Lassa virus (LASV) nucleoprotein (NP) is the only known 3′-5′ exoribonuclease that can suppress type I interferon (IFN) production possibly by degrading immune-stimulatory RNAs. NP is a multifunctional protein involved in viral genomic RNA encapsidation, viral RNA synthesis, and immune evasion. Our structural, biochemical, and cell-based analyses have demonstrated that NP encodes a functional 3′-5′ exoribonuclease of the DEDDH family at its C terminus and that this RNase activity plays a strikingly important role in IFN suppression. We therefore propose a novel immune evasion mechanism in which NP suppresses the IFN induction by selectively degrading these immune-stimulatory RNAs.

We have also conducted a time course soaking experiment to explore the kinetic process of the LASV NP exoribonuclease function. To do this, we set up a time course experiment to capture the conformational changes of the NP-C·dsRNA complex during the enzymatic reaction. The LASV NP-C·dsRNA complex was soaked in a cryoprotectant solution with 100 mm MnCl2, and the crystals were incubated for 1, 1.5, 5, or 10 min at room temperature under a standard crystallization condition but with pH 5.5 that would slow down the catalytic reaction for the purpose of capturing the different stages of the reaction. Over the time course, the crystal cell volumes changed gradually from 474,825 Å3 to 444,643 Å3. Second, the electron density of the 5′-ppp moiety of the triphosphate dsRNA substrate became clearly visible, and that of an additional nucleotide C4 at the 5′ end of the complementary strand also became partially visible. This strongly suggests that the RNA molecule identified in the NP-C·dsRNA complex structure is indeed an intermediate product of the NP-C exoribonuclease activity. In addition, the electron density for the 4-bp dsRNA in the catalytic cavity became less clear over time, which serves as evidence for the dsRNA moving toward the catalytically active site during the cleavage reaction. Last, the side chain of residue Tyr-429 became structurally disordered, whereas those of other local residues remained unchanged, indicating that the Tyr-429 residue moved from the G5 base to stack against the next C6 base of the complementary strand in the 5′ to 3′ direction (3′-CCCGXXXX-5′) when the cytidine monophosphate was removed from the 3′ end of the cleaving strand (5′-GGGC-3′).

> AMDHVEFGLTYSQLMTLKDAMLQLDPNAKTWMDIEGRPEDPVEIALYQPSSGCYIHFFREPTDLKQFKQDAKYSHGIDVTDLFATQPGLTSAVIDALPRNMVITCQGSDDIRKLLESQGRKDIKLIDIALSKTDSRKYENAVWDQYKDLCHMHTGVVVEKKKRGGKEEITPHCALMDCIMFDAAVSGGLNTSVLRAVLPRDMVFRTSTPRVVL> GSHMLNTPSGVAVDSAGTVWVTDHGNNRVVKLAAGSNTQTVLPFTGLNTPSGVAVDSAGTVWVTDHGNNRVVKLAAGSNTQTVLPFTGLN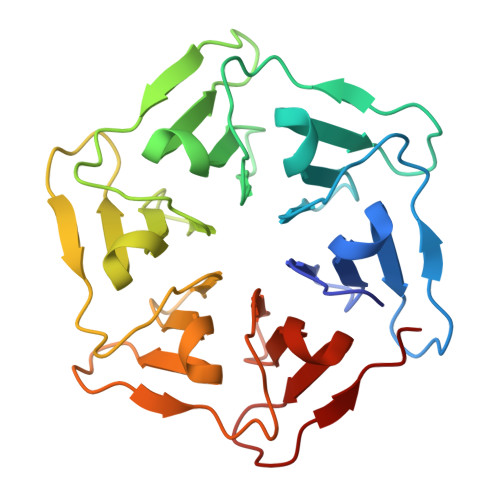TPSGVAVDSAGTVWVTDHGNNRVVKLAAGSNTQTVLPFTGLNTPSGVAVDSAGTVWVTDHGNNRVVKLAAGSNTQTVLPFTGLNTPSGVAVDSAGTVWVTDHGNNRVVKLAAGSNTQTVLPFTGLNTPSGVAVDSAGTVWVTDHGNNRVVKLAAGSNTQTVLPFT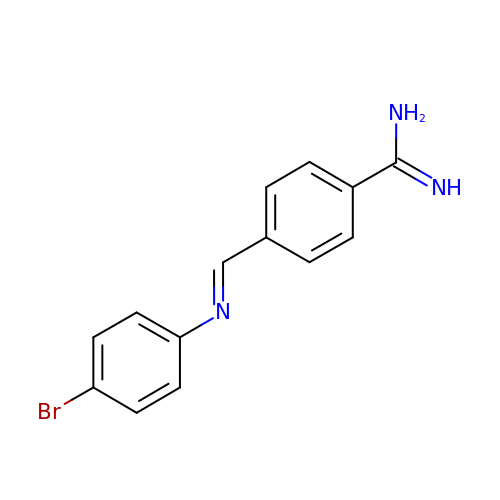(E)-4-((4-bromophenylimino)methyl)benzimidamide | C14 H12 Br N3 | JQXAHUQWUIRBGQ-GIJQJNRQSA-N>MKKLFLVFWWHMHQPLYREPYTGEYLLPWTFFHAVKDYYDMPAYLKDFEIKLNFNLTPVLIDQIQEYAQGKAKDVFLEAIRKDPDDLEKEEVEKLIEFTKLNYEKPIYRFERIRELMNKEKLNREELLDLQTLNLLAWCGRTLRKDLKDLLNKGRNYTQEEKEYVLNKYFEIIKKTLSIYREIKEEGKGSVSTSPYYHPLIPILLNPNCVYETTPNVKIPDFAVSFREDASKHVELAKEKYFEIFGEHPVYMWPPEASVSNEALELYYEKGINMLAT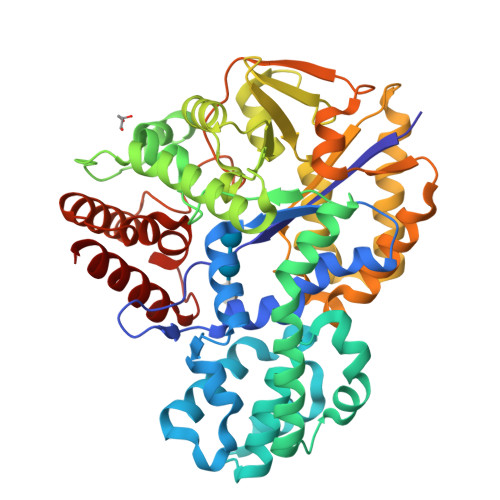DEVILKNSVERASPYLRYYFRELISVFFRDKTLSDLIGFSYHAWNAEDAVRDFIGRLKKIHESVDFQPVVFVVLDGENCWEYYEENGIPFLEKLYSTLEKEEWIETLTLEEAMRKEDVKTEVIESVKAGTWFDGNFLKWIGNKEKNEYWKILIEAKKKAKNDYILVAEGSDWFWWQGEEKAPFVEVFDKLFRSFVRRAQE[2x]>[2x]GRKRRTTVRGEGIDPEKAKSYVAPYFEKSEDETALILKLLTYNVLFSFLDSRDLMTVAGAMWRVEFKQDDCIMEAGQTTCDKLYIIQDGKADIIKEGQKVYLKVEGTAVGELELMYQTPTVATVKVCTPELIAWALDRDTYRHLVMGSAIRRRETYIQFLTNIPFLSGLDNYEKLQLADALSS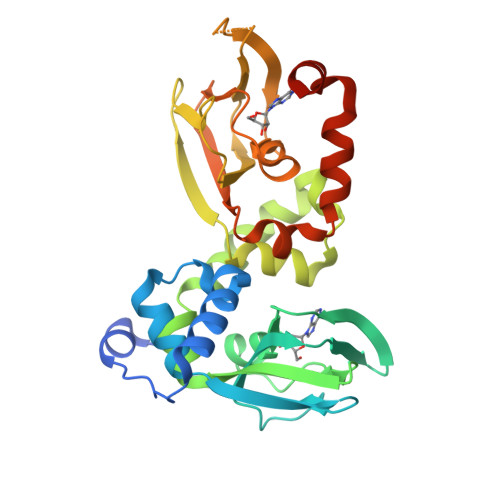DEFEPGDYIIRYGEEGEWLYIILEGSVDVVGRDDDGNEKHVWEFGKGDHVGELEFLNNHANVADVVAKTHVVTAKLNRRHFEMCLGPVIDVLKRTSQQPNYEYYQSKLKTTLRAEGRK> MLTVGFEWAAQPEKYPWMYSLPSKTEDFEDWLNQWSDFTLQWFKINKLHQISLVELMGEKPFSYLQNKSKALTVIVENLIARNFCKYTDKEYKSIRVFWRGYRDWSEVIYNWALKKGRTELTFFEIIDLKESPDNFHMLPKEDFKKIFNILVKNKRAEWINKKNMHIRILFLEHHHHHH

The ESCRT machinery, comprising of multiple proteins and subcomplexes, is crucial for membrane remodelling in eukaryotic cells, in processes that include ubiquitin-mediated multivesicular body formation, membrane repair, cytokinetic abscission, and virus exit from host cells. Metagenome assemblies of the recently discovered Asgard archaea, the closest living relatives of eukaryotes, have revealed that homologues of the entire ubiquitylation cascade, ESCRT-III (and Vps4), and components of the ESCRT-I and ESCRT-II subcomplexes are all encoded by the genomes of these archaea. In addition, we observed a consistent pattern of association across genomes in which the genes for ESCRT-III and Vps4 were found most tightly associated with homologues of Vps25. This is striking as Vps25 is the subunit of the ESCRT-II complex in eukaryotes that recruits ESCRT-III to membranes, triggering vesicle budding.

Eukaryotic ESCRT-II forms a ‘Y-shaped’ hetero-tetrameric structure consisting of a Vps22/Vps36 stalk which binds two Vps25 subunits. Structural models for the Odinarchaeotal and Hemidallarchaeotal ESCRT-II subcomplex proteins generated using AlphaFold 274,75 identified potential tandem winged helix (WH) domains, which they likely share with their eukaryotic counterparts, Vps22 and Vps2579–81. In the case of Odinarchaeotal Vps25, while we were unable to crystallize the full-length soluble protein, high-quality crystals could be generated using an N-terminally truncated version (deleting N-terminal residues 1–58), which were then used to determine the structure at a resolution of 1.80 Å. Inspection of this structure revealed that the Asgard Vps25 core is composed of a tandem WH domain repeat, consistent with the predicted AlphaFold 2 model. B Superposition of the N- (blue) and C-terminal (wheat) Asgard Vps25 WH domains demonstrating their similarity. The alignment shown superimposes the N-terminal WH domains, only, and yields all-atom RMSD values against the Odin N-terminal WH domain of 0.7 Å and 1.1 Å for the yeast and human N-terminal WH domains, respectively. A similar alignment of the C-terminal WH domains yielded all-atom RMSD values of 1.5 Å and 1.1 Å for the yeast and human domains against the Odin C-terminal WH domain. Because of changes in the relative orientations of the WH domains with respect to each other in the tandem arrangement of the three Vps25 homologues, overall alignment gives much higher all-atom RMSD values of 3.5 Å and 5.1 for the yeast and human proteins against Odin, respectively. The same appears to be true for the Asgard ESCRT-II machinery which, based upon modelling of Vps22 and Vps25 proteins from Odinarchaeota and the crystallographic Odinarchaeotal Vps25 structure, possess two very similar WH domains. This suggests that all ESCRT-II proteins were initially derived from a single-WH domain protein progenitor, with Vps36 emerging during eukaryogenesis.> MSLHYQPKQDLLQNRIILVTGASDGIGREAALTYARYGATVILLGRNEEKLRR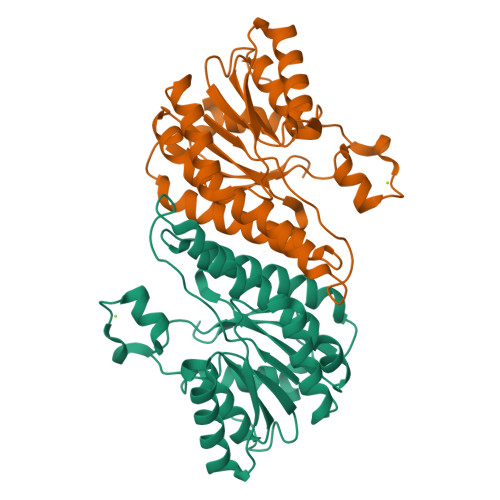VAQHIADEQHVQPQWFTLDLLTCTAEECRQVADRIAAHYPRLDGVLHNAGLLGEIGPMSEQDPQIWQDVMQVNVNATFMLTQALLPLLLKSDAGSLVFTSSSVGRQGRANWGAYATSKFATEGMMQVLADEYQNRSLRVNCINPGGTRTSMRASAFPTEDPQKLKTPADIMPLYLWLMGDDSRRKTGMTFDAQPGRKEGHHHHHH>[6x]GSHMRESAEEVWGGTEDLTSLSVEELKGLMARFDEEEKRISYRRRVMQGRIDVIRA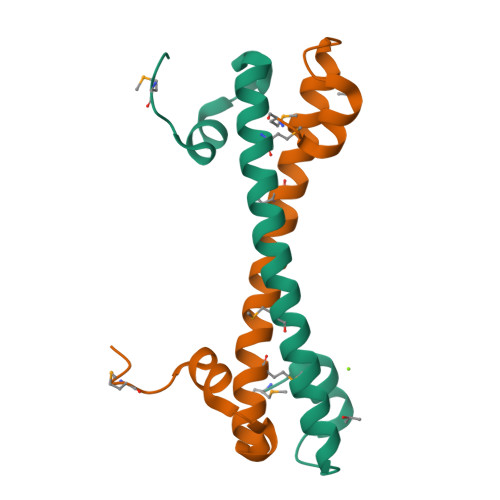EIVRRGGAVLSPEELARVLMGDVGDESE> AHHH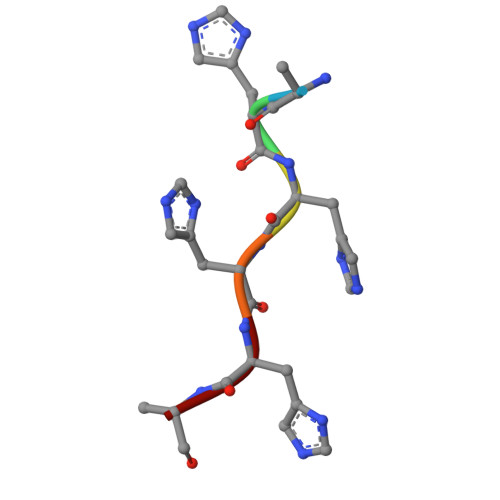HA> MTTRLTRWLTALDNFEAKMALLPAVRRYGRLTRATGLVLEATGLQLPLGATCIIERQDGPETKEVESEVVGFNGQRLFLMPLEEVEGILPGARVYARNGHGDGLQSGKQLPLGPALLGRVLDGGGKPL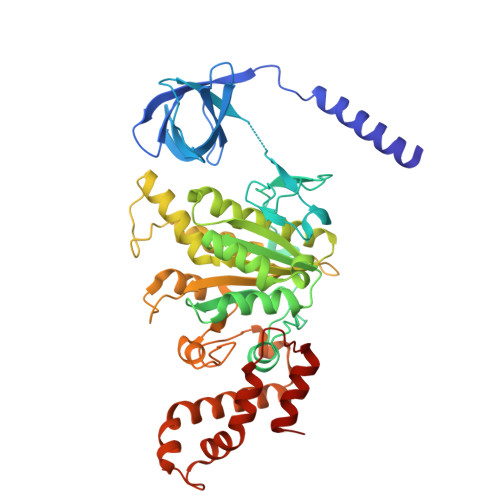DGLPAPDTLETGALITPPFNPLQRTPIEHVLDTGVRAINALLTVGRGQRMGLFAGSGVGKSVLLGMMARYTRADVIVVGLIGERGREVKDFIENILGPDGRARSVVIAAPADVSPLLRMQGAAYATRIAEDFRDRGQHVLLIMDSLTRYAMAQREIALAIGEPPATKGYPPSVFAKLPALVERAGNGIHGGGSITAFYTVLTEGDDQQDPIADSARAILDGHIVLSRRLAEAGHYPAIDIEASISRAMTALITEQHYARVRLFKQLLSSFQRNRDLVSVGAYAKGSDPMLDKAITLWPQLEAFLQQGIFERADWEDSLQALDLIFPTV>[4x]MAIEFTKYHGLGNDFILIDNRASKTPAITPEKAVEMCDRHFGIGADGVIFALPGENGTDYTMRIFNSDGSEPEMCGNGIRCLAAFLADLEGLSRNKDTYRIHTLAGVITPQLTPDGQIKVDMGLPRLLAGEIPTNIAAADQKVINQPLEVEGKTWEVTCVSMGNPHCITFVEDVAAIPLETIGPKFEHHPAFPQRTNTEFIQVVSRDYLKMRVWERGAGITLA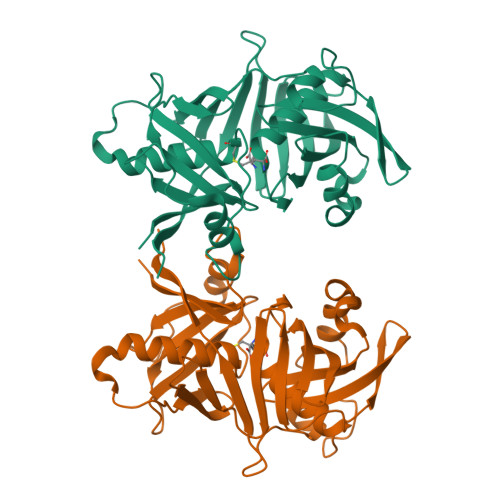CGTGACASLVAAVLTGRSDRLATVELPGGPLEIEWSEVDQRIYMTGPADRVFTGKLHHHHHH N-{5-[(2-{[3,5-difluoro-4-(1-methylpiperidin-4-yl)phenyl]amino}-5-methylpyrimidin-4-yl)amino]-2-fluorophenyl}-2-methylpropane-2-sulfonamide | C27 H33 F3 N6 O2 S | 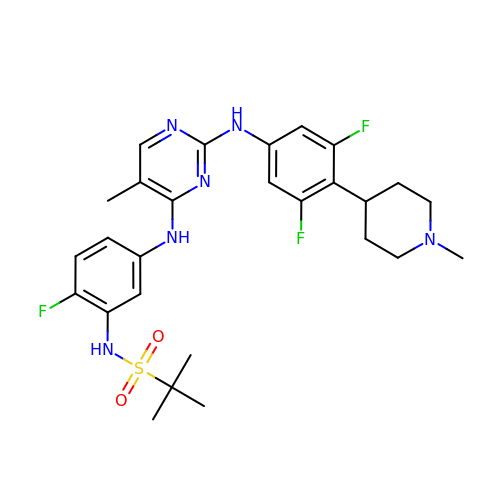YJTYYXRVQGLUFN-UHFFFAOYSA-N>MRKMQDYKFWFVVGSQPLYGPEALAEVEKDARKLVDGLNKGGKLDYPVEFKLVATTADSITKFMKEANYNDDVAGVITWMHTFSPAKNWIRGTELLQKPLLHLATQFLNNIPFDSIDMDYMNLHQSAHGDREYAYINSRLNVPAASVYGWWGDADVQEQIADWQHVAVAYNESFHIKIARFGDTMRDVAVTEGDKVAAQIKLGWTVDYYPTNELVAVVNGIAEDEIDAAYKDLEANYDLVEGDNDHEKYVHNVRYQLREYLGIKKFLDDNGYDAFTDNFQDLEGLEQLPGLAVQLLMIDGYGFGPEGDFKMAGLTRLLKIAADNKQTALMEDYT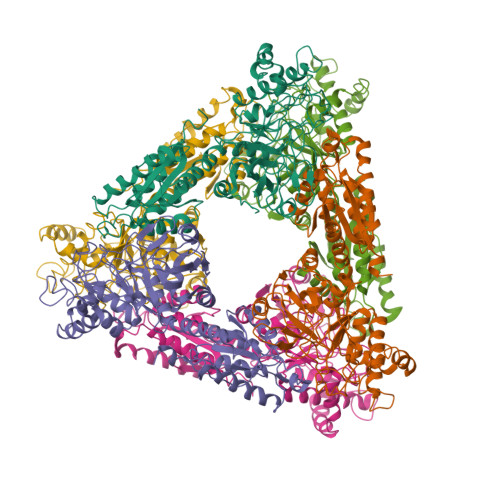LDLRHGHEAIMGSHMLEVDPTLASDKPRVEVHPLGIGGKDDPARLVFTGAEGKGYDITLSYFDDGYKFIGYPVDCKTPEAEMPKLPVAKQMWTPEIGLAEGAKQWMKYGGGHHTVLTLALSEEQLEQLARLFKVDFINIK[6x]6-methylhept-5-en-2-one 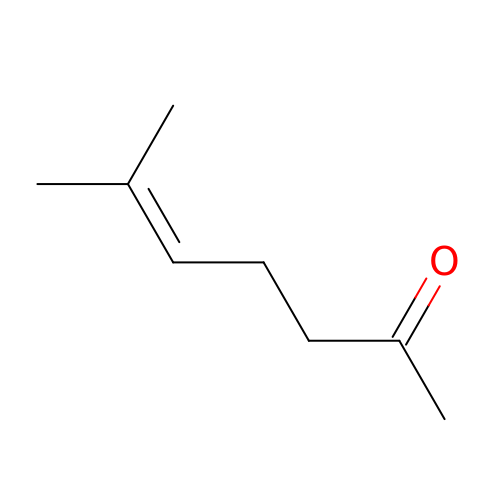| C8 H14 O | UHEPJGULSIKKTP-UHFFFAOYSA-N>GPGSGKNKVRRVKTIYDCQADNDDELTFIEGEVIIVTGEEDQEWWIGHIEGQPERKGVFPVSFVH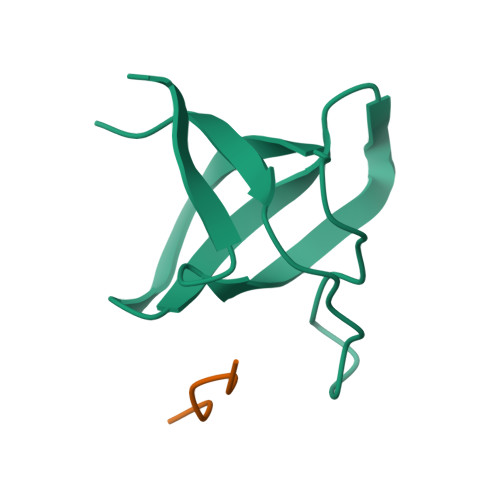ILSD[4x];>[4x]GIKKPVRRKLKE[1-(4-FLUOROBENZYL)CYCLOBUTYL]METHYL (1S)-1-[OXO(1H-PYRAZOL-5-YLAMINO)ACETYL]PENTYLCARBAMATE | C23 H29 F N4 O4 | 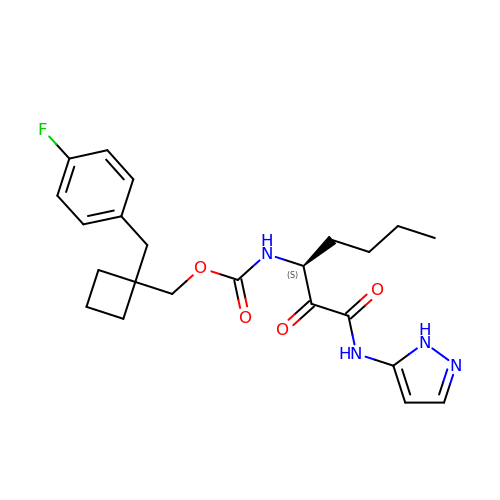QTPYRNAKLBXKNP-SFHVURJKSA-N> SEISRQEFQRRRQALVEQMQPGSAALIFAAPEVTRSADSEYPYR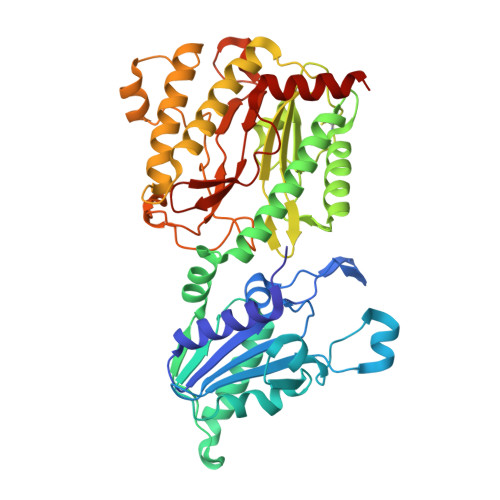QNSDFWYFTGFNEPEAVLVLIKSDDTHNHSVLFNRVRDLTAEIWFGRRLGQDAAPEKLGVDRALAFSEINQQLYQLLNGLDVVYHAQGEYAYADVIVNSALEKLRKGSRQNLTAPATMIDWRPVVHEMRLFKSPEEIAVLRRAGEITAMAHTRAMEKCRPGMFEYHLEGEIHHEFNRHGARYPSYNTIVGSGENGCILHYTENECEMRDGDLVLIDAGCEYKGYAGDITRTFPVNGKFTQAQREIYDIVLESLETSLRLYRPGTSILEVTGEVVRIMVSGLVKLGILKGDVDELIAQNAHRPFFMHGLSHWLGLDVADVGVYGQDRSRILEPGMVLTVEPGLYIAPDAEVPEQYRGIGIRIEDDIVITETGNENLTASVVKKPEEIEALMVAARKQ3,5-bis(bromanyl)-4-oxidanyl-benzoic acid | C7 H4 Br2 O3 | 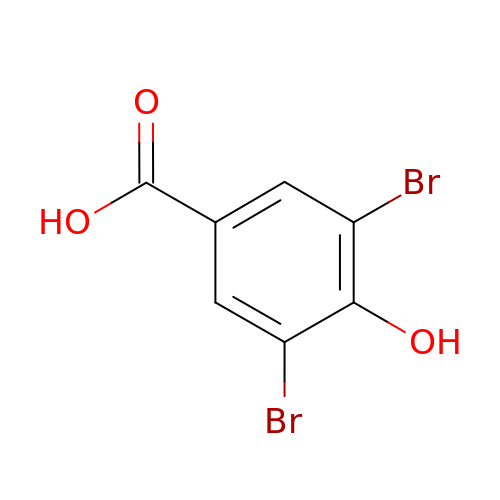PHWAJJWKNLWZGJ-UHFFFAOYSA-N>RWTGRQKARGAATRARQKQRASLETMDKAVQRFRLQNPDLDSEALLTLPLLQLVQKLQSGELSPEAVFFTYLGKAWEVNKGTNCVTSYLTDCETQLSQAPRQGLLYGVPVSLKECFSYKGHDSTLGLSLNEGMPSESDCVVVQVLKLQGAVPFVHTNVPQSMLSFDCSNPLFGQTMNPWKSSKSPGGSSGGEGALIGSGGSPLGLGTDIGGSIRFPSAFCGICGLKPTGNRLSKSGLKGCVYGQTAVQLSLGPMARDVESLALCLKALLCEHLFTLDPTVPPLPFREEVYRSSRPLRVGYYETDNYTMPSPAMRRALIETKQRLEAAGHTLIPFLPNNIPYALEVLSAGGL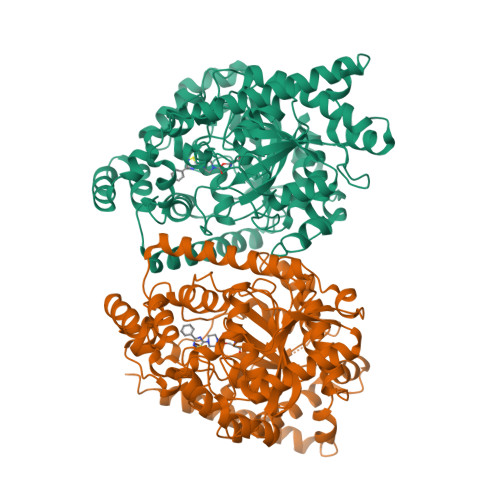FSDGGRSFLQNFKGDFVDPCLGDLILILRLPSWFKRLLSLLLKPLFPRLAAFLNSMRPRSAEKLWKLQHEIEMYRQSVIAQWKAMNLDVLLTPMLGPALDLNTPGRATGAISYTVLYNCLDFPAGVVPVTTVTAEDDAQMELYKGYFGDIWDIILKKAMKNSVGLPVAVQCVALPWQEELCLRFMREVEQLMTPQKQPS[2x]Previous studies have confirmed that the B318L protein encoded by the ASFV represents a new member of the viral PT family, according to sequence alignment and a follow-up enzymatic assay. These experiments have shown that the B318L protein catalyzes the condensation of isopentenyl diphosphate (IPP) with allylic diphosphates to produce C20-geranylgeranyl diphosphate (GGPP) and longer chain prenyl diphosphates. Taken together, these experiments indicate that B318L is an essential gene for viral replication.

For crystallization, the N-terminal putative transmembrane region (residues 1–30) was truncated. Thus, the truncated form of B318L (residues 31–318) was expressed in E. coli. In this study, taking advantage of an accurate model predicted from AF2, the crystal structure of the B318L protein was successfully solved by MR at 3.2 Å. The overall structure of B318L adopts a canonical all-helix fold and contains 11 helices (A to K) which can be divided into three layers. The front helical layer is formed by helices A, B, and E. The front layer is orthogonal to the other layers. In the middle layer, there are helices C, D, F, I, and K. The conserved Asp-rich motifs FARM (residues 129–135) and SARM (residues 257–261) are located at helices D and I, respectively. The remaining helices G, H, and J, surrounding the catalytic core, form the back layer. However, there are three loop regions (S133 to K143, Q209 to P214, and H262 to N269) that could not be built due to the lack of interpretable electron density. The most significant difference is the various conformations of their N-terminal extensions, where the N-terminus of B318L starts with a long loop, whereas helices are observed in the N-terminus of other GGPPS. Since the experimental structure inherently belongs to the apo form of the B318L protein, its protein-ligand contact area is much closer to the apo templates.

> APRSVALFHGIHPLNPKNYKTFSKEFETILNNAIEDGDFKGQLTEPCSYALRGGKYIRPIILMEIVRACQLQHSFGAPIYPAEAALAVEYFHVASLIIDDMPSFDNDVKRRNKDTVWARFGVAKAQMSALALTMQGFQNICRQIDWIKEHCPRFPDPNQLGALLCTFVSHSLNSAGSGQLVDTPEKTIPFFKIAFIMGWVLGTGTIEDIGMIERAAHCFGHAFQLADDIKDHDTDTGWNYAKIHGKQKTFDDVAQSLQECKKILHGKKIFTSIWNEIFQKVINVALGT~{N}-[4-(6,7-dimethoxyquinazolin-4-yl)oxyphenyl]-2-(4-propan-2-yl-1,2,3-triazol-1-yl)ethanamide | C23 H24 N6 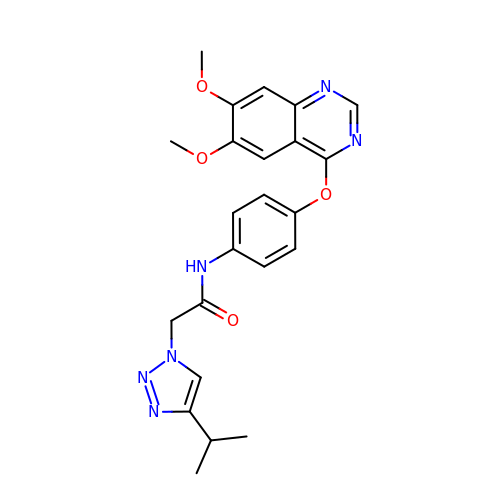O4 | VOSCKXNNVDOPMN-UHFFFAOYSA-N5-(2,5-DICHLOROPHENYL)-2-FUROIC ACID | C11 H6 Cl2 O3 | 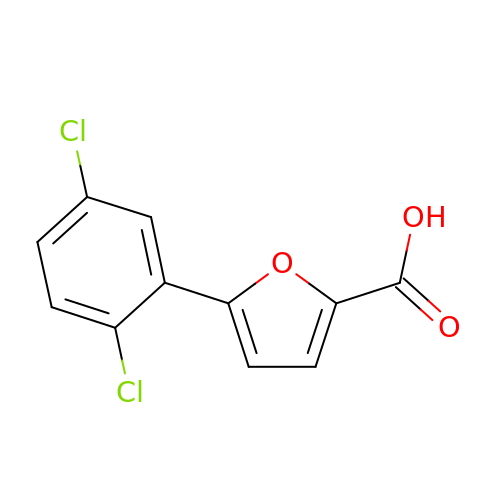ATAZLMGGQQLRBC-UHFFFAOYSA-N> RGPA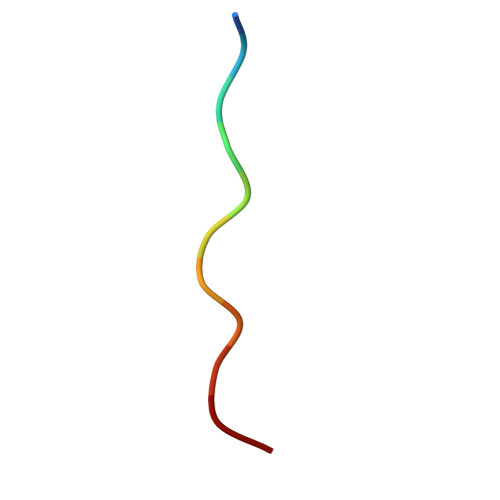PPPPPHR>MKNLTTIKQTNKNVKQERRKKYADLAIQGTNNSSIASKRSVELLYLPKLSSANNFQMDKNNKLLEYFKFFVPKKIKRSPCINRGYWLRLFAIRSRLNSIIEQTPQDKKIVVVNLGCGYDPLPFQLLDTNNIQSQQYHDRVSFIDIDYSDLLKIKIELIKTIPELSKIIGLSEDKDYVDDSNVDFLTTPKYLARPCDLNDSKMFSTLLNECQLYDPNVVKVFVAEVSLAYMKPERSDSIIEATSKMENSHFIILEQLIPKGPFEPFSKQMLAHFKRNDSPLQSVLKYNTIESQVQRFNKLGFAYVNVGDMFQLWESADEATKKELLKVEPFDELEEFHLFCHHYVLCHATNYKEFAFTQGFLFDRSISEINLTVDEDYQLLECECPINRKFGDVDVAGNDVFYMGGSNPYRVNEILQLSIHYDKIDMKNIEVSSSEVPVARMCHTFTTISRNNQLLLIGGRKAPHQGLSDNWIFDMKTREWSMIKSLSHTRFRHSACSLPDGNVLILGGVTEGPAMLLYNVTEEIFKDVTPKDEFFQNSLVSAGLEFDPVSKQGIILGGGFMDQTTVSDKAIIFKYDAENATEPITVIKKLQHPLFQRYG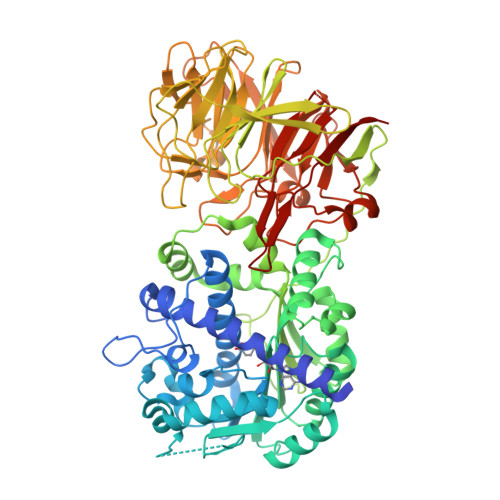SQIKYITPRKLLIVGGTSPSGLFDRTNSIISLDPLSETLTSIPISRRIWEDHSLMLAGFSLVSTSMGTIHIIGGGATCYGFGSVTNVGLKLIAIAK[2x]> SLRPKLSEEQQRIIAILLDAHHKTYDPTYSDFCQFRPPVRVNDGGGSVTLELLQLSMLPHLADLVSYSIQKVIGFAKMIPGFRDLTSEDQIVLLKSSAIEVIMLRSNESFTMDDMSWTCGNQDYKYRVSDVTKAGHSLELIEPLIKFQVGLKKLNLHEEEHVLLMAICIVSPDRPGVQDAALIEAIQDRLSNTLQTYIRCRHPPPGSHLLYAKMIQKLADLRSLNEEHSKQYRCLSFQPECSMKLT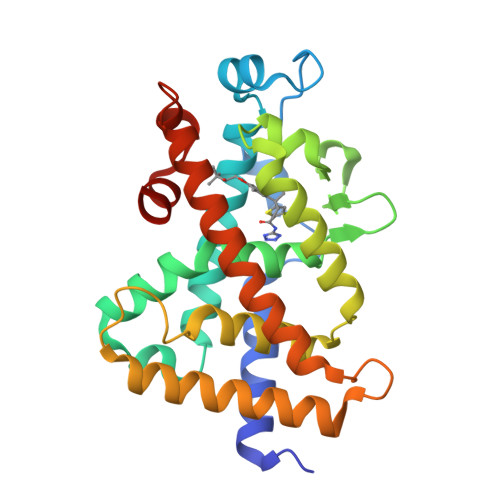PLVLEVFGNEG>RTPEMPVLENRAAQGDITAPGGARRLTGDQTAALRDSLSDKPAKNIILLIGDGMGDSEITAARNYAEGAGGFFKGIDALPLTGQYTHYALNKKTGKPDYVTDSAASATAWSTGVKTYNGALGVDIHEKDHPTILEMAKAAGLATGNVSTAELQDATPAALVAHVTSRKCYGPSATSEKCPGNALEKGGKGSITEQLLNARADVTLGGGAKTFAETATAGEWQGKTLREQAQARGYQLVSDAASLNSVTEANQQKPLLGLFADGNMPVRWLGPKATYHGNIDKPAVTCTPNPQRNDSVPTLAQMT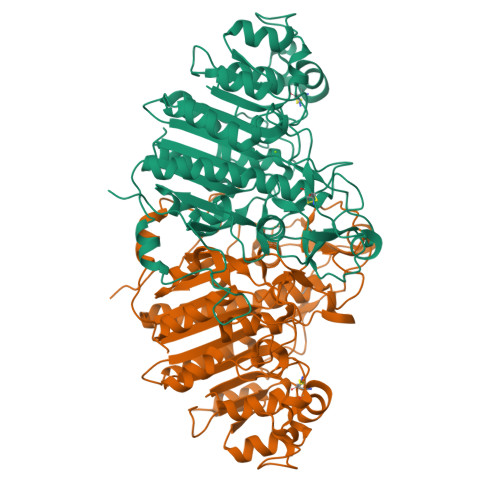DKAIELLSKNEKGFFLQVEGASIDKQDHAANPCGQIGETVDLDEAVQRALEFAKKEGNTLVIVTADHAHASQIVAPDTKAPGLTQALNTKDGAVMVMSYGNSEEDSQEHTGSQLRIAAYGPHAANVVGLTDQTDLFYTMKAALGLKLEHHHHHH[2x]>[2x]MSHSSAPERATGAVITDWRPEDPAFWQQRGQRIASRNLWISVPCLLLAFCVWMLFSAVAVNLPKVGFNFTTDQLFMLTALPSVSGALLRVPYSFMVPIFGGRRWTAFSTGILIIPCVWLGFAVQDTSTPYSVFIIISLLCGFAGANFASSMANISFFFPKQKQGGALGLNGGLGNMGVSVMQLVAPLVVSLSIFAVF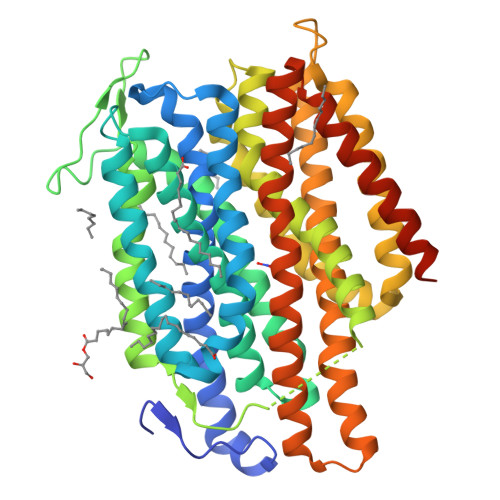GSQGVKQPDGTELYLANASWIWVPFLAIFTIAAWFGMNDLATSKASIKEQLPVLKRGHLWIMSLLYLATFGSFIGFSAGFAMLSKTQFPDVQILQYAFFGPFIGALARSAGGALSDRLGGTRVTLVNFILMAIFSGLLFLTLPTDGQGGSFMAFFAVFLALFLTAGLGSGSTFQMISVIFRKLTMDRVKAEGGSDERAMREAATDTAAALGFISAIGAIGGFFIPKAFGSSLALTGSPVGAMKVFLIFYIACVVITWAVYGRHSKKLESSGENLYFQG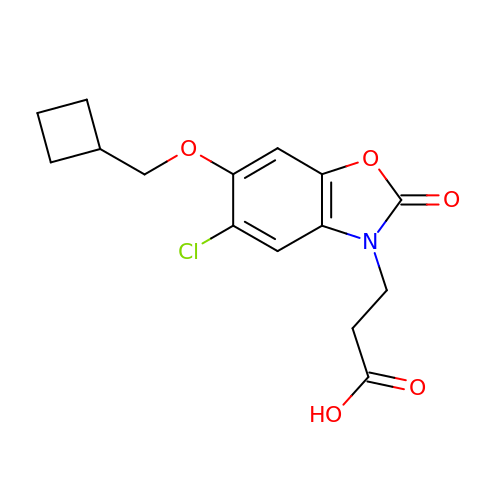3-[5-chloro-6-(cyclobutylmethoxy)-2-oxo-2,3-dihydro-1,3-benzoxazol-3-yl]propanoic acid | C15 H16 Cl N O5 | VZSAISDQEBTHJE-UHFFFAOYSA-N> GSAQADFDIPAGPLAPALAHFGQSAHILLSYPTALTEGRSTSGLAGRFDIDQGLAILL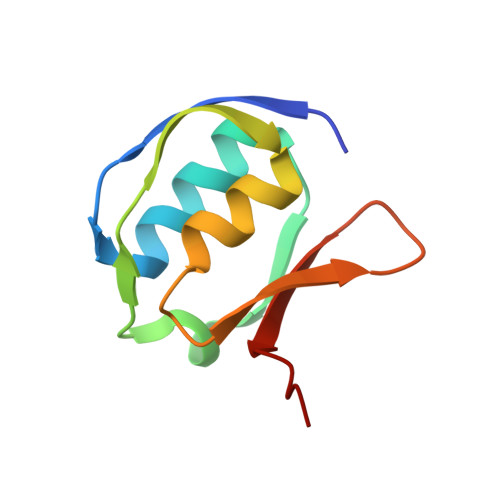AGTGLEASRGANASYSLQASASTG> NLSLSQSNFSADTYKSFIKNLRKQLTIGASYGSAGIPILKHSVP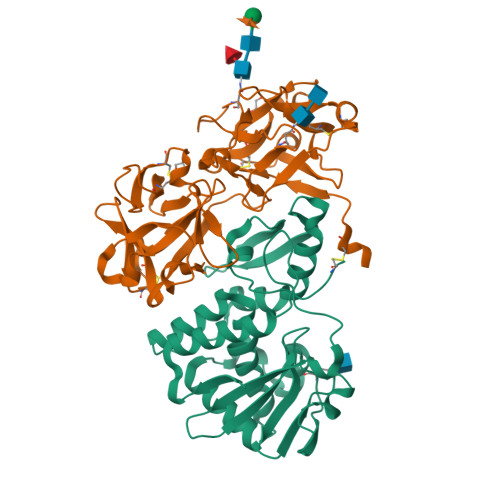ICERFLLVDLTNGDNETITLAINVEDAGFAAYRAADRSYFFQNAPPIASYVIFTDTNQNIMNFNNTFESIEIVGGTTRSETPLGIMHFEASIFHLFVHDENYVPTSFLVLIQMVLEAAKFKFIEQKVIHSIMDMEDFTPGLAMLSLEENWTQLSLQLQASESLNGVFGDSVSLYNSMDEPIGVDSMYYPILTANMAFQLYQCP;> NEQCSPQQRTTRISGRDGLCVDVYGALTADGSRVILYPCGQQQNQQWTFYPDNTIRSLGKCLATSALSSGSNVVITNCDYLRYDDGWMVSSSGTMMNKSSHLVLTANAATSRTNLTGENNVFAAKQAWRIGNYVEPIVTTIIGLRHMCLEATDNDTNVWLESCVKNKTKQYWALYSDDTIRVNNNRNLCVSSSTDSSSKLIVIRRCDGSINQRWVFTPQGTISNPGYEAVMDVAQNDVYLKKIVLSSATDKGNGQQWTVFY> SMEQPEPDMITIFIGTWNMGNAPPPKKITSWFLSKGQGKTRDDSADYIPHD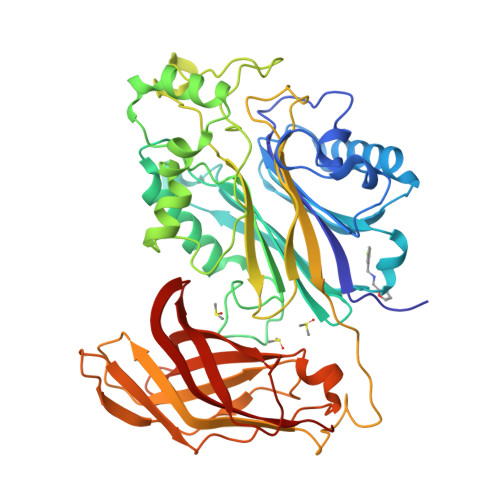IYVIGTQEDPLSEKEWLEILKHSLQEITSVTFKTVAIHTLWNIRIVVLAKPEHENRISHICTDNVKTGIANTLGNKGAVGVSFMFNGTSLGFVNSHLTSGSEKKLRRNQNYMNILRFLALGDKKLSPFNITHRFTHLFWFGDLNYRVDLPTWEAETIIQKIKQQQYADLLSHDQLLTERREQKVFLHFEEEEITFAPTYRFERLTRDKYAYTKQKATGMKYNLPSWCDRVLWKSYPLVHVVCQSYGSTSDIMTSDHSPVFATFEAGVTSQFVSKNGPGTVDSQGQIEFLRCYATLKTKSQTKFYLEFHSSCLESFVKSQEGENEEGSEGELVVKFGETLPKLKPIISDPEYLLDQHILISIKSSDSDESYGEGCIALRLEATETQLPIYTPLTHHGELTGHFQGEIKLQTSQ The most prominent such domain has been identified by bioinformatics as part of non-structural protein 3 (Nsp3) of the virus and appropriately named the “SARS-unique domain” (SUD). SUDcore turns out to consist of two subdomains, SUD-N (Nsp3 residues 389–517) and SUD-M (525–652), each exhibiting the fold of a macrodomain. The two subdomains are connected by a flexible linker (residues 518–524) and a disulfide bond. Instead, we have demonstrated that full-length SUD and SUDcore bind oligodeoxynucleotides and oligoribonucleotides that form G-quadruplexes.

In this communication, we describe the crystal structures at 2.2 Å and 2.8 Å resolution (monoclinic and triclinic form, respectively) of the core of the SARS-unique domain (SUDcore, Nsp3 residues 389–652). Two crystal forms were observed under identical crystallization conditions: Form-1 crystals were monoclinic (space group P21, two SUDcore molecules per asymmetric unit) and diffracted X-rays to 2.2 Å resolution; form-2 crystals were triclinic (space group P1, four SUDcore molecules per asymmetric unit) and diffracted to 2.8 Å. Both structures were determined by molecular replacement. The r.m.s. deviations (on Cα atoms) between the models derived from the two different crystal structures are around 0.7 Å. In both crystal forms, SUDcore displays the same head-to-tail dimer, with the SUD-N subdomain of monomer A interacting with the SUD-M subdomain of monomer B, and vice versa. Due to the two-domain architecture of each monomer, the resulting four lobes give the dimer a quasi-tetrahedral shape. As to be expected, the structures of the monomers are very similar to one another, with r.m.s.d. values (for Cα atoms) of 0.58 Å between monomers A and B of the monoclinic crystal form, and 0.11–0.37 Å between monomers A–D of the triclinic form. In all six independent copies of the SUDcore monomer, residue Val611 adopts forbidden conformational angles. The side chain makes a hydrophobic contact across the subdomain interface and is also contacting the side chain of Phe406 of a symmetry-related SUDcore dimer in the crystal lattice in the monoclinic crystal form (this also applies to two of the four monomers in the triclinic form). One potential binding site for G-quadruplexes might be in a cleft between two consecutive SUDcore dimers as they occur in both the monoclinic and triclinic crystal forms, but for confirmation, any of these models will have to await crystallographic determination of the complex.

>KIKACIDEVTTTLEETKFLTNKLLLFADINGKLYHDSQNMLRGEDMSFLEKDAPYMVGDVITSGDITCVVIPSKKAGGTTEMLSRALKKVPVDEYITTYPGQGCAGYTLEEAKTALKKCKSAFYVLPSEAPNAKEEILGTVSWNLREMLAHAEETRKLMPICMDVRAIMATIQRKYKGIKIQEGIVDYGVRFFFYTSKEPVASIITKLNSLNEPLVTMPIGYVTHGFNLEEAARCMRSLRAPAVVSVSSPDAVTTYNGYLTSSS[4x]> VNSVTISVEGMTCNSCVWTIEQQIGKVNGVHHIKVSLEEKNATIIYDPKLQTPKTLQEAIDDMGF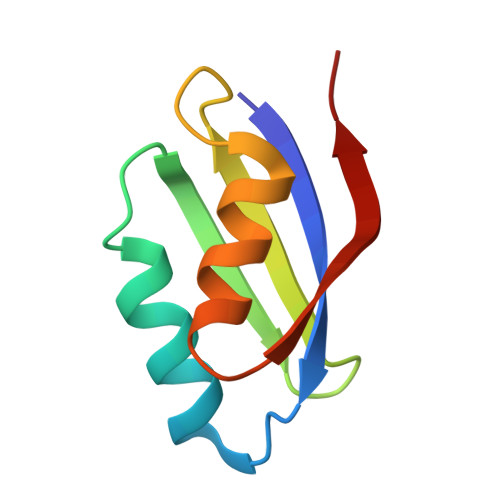DAVIHNIEGR The Munc13–1/α-RIM interaction is particularly interesting in this regard since its physiological importance has been demonstrated and both Munc13–1 and α-RIMs are involved in priming and plasticity. Our results suggest that a Munc13–1 homodimer–Munc13–1/α-RIM heterodimer switch regulates neurotransmitter release and some forms of presynaptic plasticity, and reveal the structural basis for homo- and heterodimerization. 2A domain can in fact establish two different types of interactions that lead to either homodimerization with itself or heterodimerization with the RIM2α ZF domain. Since the Munc13–1/α-RIM interaction competes with Munc13–1 homodimerization, this model predicts that Munc13–1 may exist in solution as a homodimer that needs to be disrupted in order to bind to α-RIMs at the active zone.

2A-domain homodimer at 1.44 Å resolution, designed a mutation that disrupts homodimerization, and solved the X-ray crystal structure at 1.78 Å resolution of a Munc13–1 fragment bearing this mutation bound to the RIM2α ZF domain. The X-ray structure of the Munc13–1/RIM2α heterodimer described here provides the first high-resolution view of a complex directly involving a member from the family of ZF domains that includes α-RIMs and other Rab effectors. 2A domain and the α-helix with opposite sites of the ZF domain. 2A domain and the C-terminal α-helix exhibit an overt shape complementarity. 2A domain and C-terminal α-helix packs well against the ZF domain. 2A domain arising from the expression vector used also extends across to make contacts with strand 3 of the ZF-domain, but otherwise is not well packed against it. 82–142 observed in the crystals is consistent with all available data obtained in solution, whereas that involving monomer B is not. Thus, NMR studies showed that a long α-helix (helix a1) and an SGAWFY motif at the end of the short α-helix at the C-terminus of the RIM2α ZF domain (helix a2) bind to Rab3A, and that the interaction involving the SGAWFY motif is released upon binding of Munc13–1 to the ZF domain. 2A domain would have steric clashes with Rab3A upon binding to RIM2α. An emerging theme from these observations is that, because of their small size, ZF domains may often use multiple surfaces to increase the affinity and specificity of interactions with target proteins, although further research will be necessary to assess the generality of this notion.

>GSPGISGGGGGILSLLCVGVKKAKFDGAQEKFNTYVTLKVQNVESTTIAVRGSQPSWEQDFMFEINRLDLGLTVEVWNKGLIWDTMVGTVWIPLRTIRQSNEEGPGEWLTLDSQAIMADSEICGTKDPTFHRILLDAHFELPLDIPEEEARYWAKKLEQLNAKLNSS[2x];> GSQEQKGDAPTCGICHKTKFADGCGHNCSYCQTKFCARCGGRVSLRSNKVMWVCNLCRKQQE>[2x]VFHKIRNEDLIFNESLGQGTFTKIFKGVRREVGDYGQLHETEVLLKVLDKAHRNYSESFFEAASMMSKLSHKHLVLNYGVCFCGDENILVQEFVKFGSLDTYLKKNKNCINILWKLEVAKQLAAAMHFLEENTLIHGNVCAKNILLIREEDRKTGNPPFIKLSDPGISITVLPKD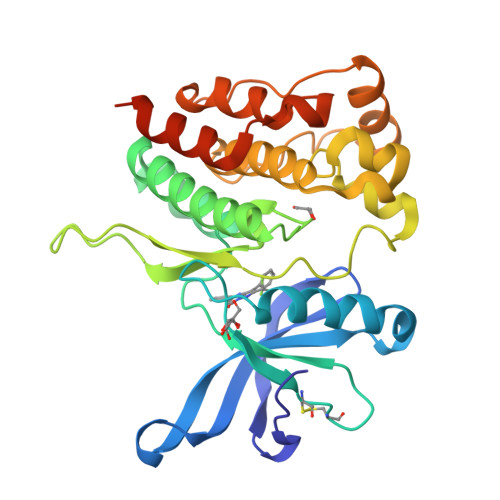ILQERIPWVPPECIENPKNLNLATDKWSFGTTLWEICSGGDKPLSALDSQRKLQFYEDRHQLPAPKAAELANLINNCMDYEPDHRPSFRAIIRDLNSLFTPDLVPRGSHHHHHH>MRRTTKETDIIVEIGKKGEIKTNDLILDHMLTAFAFYLGKDMRITATYDLRHHLWEDIGITLGEALRENLPEKFTRFGNAIMPMDDALVLVSVDISNRPYANVDVNIKDAEEGFAVSLLKEFVWGLARGLRATIHIKQLSGENAHHIVEAAFKGLGMALRVATKESERVESTKGVL[3x]

The program of herbicide development described herein aims to identify inhibitors of imidazoleglycerolphosphate‐dehydratase (IGPD; EC 4.2.1.19), an enzyme of histidine biosynthesis in plants and microorganisms. This enzyme catalyzes the manganese(II)‐dependent dehydration of (2R,3S)‐2,3‐dihydroxy‐3‐(1H‐imidazol‐5‐yl)propyl dihydrogen phosphate (2R,3S‐IGP) to 3‐(1H‐Imidazol‐4‐yl)‐2‐oxopropyl dihydrogen phosphate (IAP).4 IGPD shows strict enantioselectivity for its substrate, with the other three diastereoisomers of IGP acting as competitive inhibitors of the enzyme, thus indicating that the active site shows some flexibility to accommodate inverted chiral centers. Previous studies have shown that IGPD is inhibited by triazolylphosphonates, whose potency is based on mimicking key reaction intermediates. In this paper we describe work on the lead compound, 2‐hydroxy‐3‐(1,2,4‐triazol‐1‐yl) propylphosphonate (C348) and present a series of structures of IGPD, from Arabidopsis thaliana, complexed with a synthetic racemate of C348 and with the enantiopure compounds.

Significantly, the mirror‐image packing of the two enantiomers of C348 in IGPD2 gives rise to equipotency and, as in d/l‐AOPP superinhibitors of phenylalanine ammonia‐lyase, the mimicry of a reaction intermediate gives rise to potent inhibition. This study adds to the ever‐growing body of evidence that certain enzymes are chirally promiscuous and that mirror‐image packing of ligands is a more common feature than is generally recognized in the field of drug development.>[4x]GSHMRIAQVAPLWERVPPPAYGGVELVVSLLTEELVKRGHEVTLFASGDS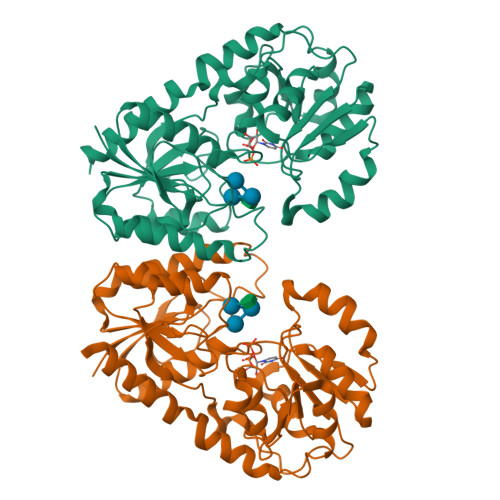MTQAKLVSTYPHAIRLDPNVQEYAVYEALQLGEVFSRANEFDVIHSHVGYTALPYTSLVKTPVVHTLHGRFTADNERIFSQYRNQNYVSISHSQRQLRELNYIATVYNAIAVETHHFYPQPSDPPYLAFLGRLSPEKGPHHAIEIAKRVGIPLRMAGKVDRVDRDYFKELIEPHIDGEFIQFIGEADHPTKNALLGGAIAMLFPITWQEPFGLVMIESMAAGTPVVAIAKGAAPEVIEHGKTGFLCHSVEDCVAAVAQVPQLDRMACRDYVWQRFSVERMVSEYEAVYDTVLANT> MEMWLRQAEDRFRFPVFPSSFSINGKAAVNSSSILKIGEIATFGGVALKSISISSFFPNKDYTFCDYTGFPSPYDCVNKIEKWMKEGFILRFTITETNINMEVIIEG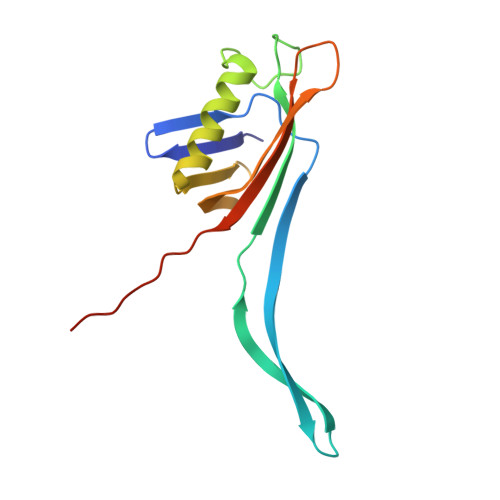FSYEERDGTRDVYFTLDLKEYKRIKIPKVTPKQ> GHMAVPDDDDDDDNSNDESEYESSQMDSEKNKGSIKNSKNVVIYADGVYDMLHLGHMKQLEQAKKLFENTTLIVGVTSDNETKLFKGQV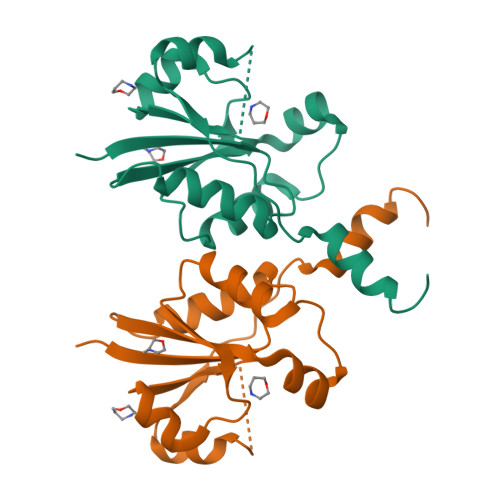VQTLEERTETLKHIRWVDEIISPCPWVVTPEFLEKYKIDYVAHDDIPYANNQKEDIYAWLKRAGKFKATQRTEGVSTTDLIVRILKNYED> GSGVEGLPSGSALLVVKRGPNAGSRFLLDQ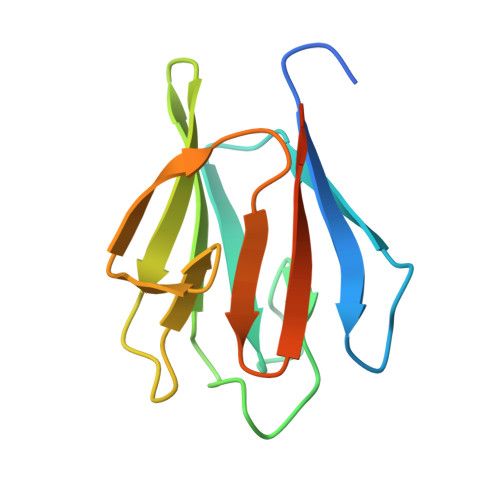PTTSAGRHPDSDIFLDDVTVSRRHAEFRLEGGEFQVVDVGSLNGTYVNREPVDSAVLANGDEVQIGKFRLVFLTGPKSDDSGSNA> MSSDYVMATKDGRMILTDGKPEIDDDTGLVSYHDQQGNAMQINRDDVSQII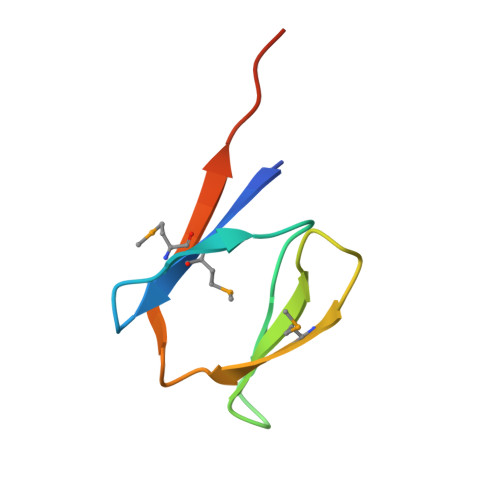ERLEHHHHHH> GSKNIVNTSILSIVYKKDDLIDLSRYGAKINIGDRVYYDSIDKNQIKLINLESSTIEVILKNAIVYNSMYENFSTSFWIKIPKYFSKINLNNEYTIINCIENNSGWKVSLNYGEIIWTLQDNKQNIQRVVFKYSQMVNISDYINRWIFVTITNNRLTKSKIYINGRLIDQKPISNLGNIHASNKIMFKLDGCRDPRRYIMIKYFNLFDKELNEKEIKDLYDSQSNSGILKDFWGNYLQYDKPYYMLNLFDPNKYVDVNNIGIRGYMYLKGPRGSVVTTNIYLNSTLYEGTKFIIKKYASGNEDNIVRNNDRVYINVVVKNKEYRLATNASQAGVEKILSALEIPDVGNLSQVVVMKSKDDQGIRNKCKMNLQDNNGNDIGFIGFHLYDNIAKLVASNWYNRQVGKASRTFGCSWEFIPVDDGWGESSL;> MKKHHHHHHGSLVPRGSDVIKPLQSDEYALLTRNVERDKYANFTINFTMENQIHTGMEYDNGRFIGVKFKSVTFKDSVFKSCTFEDVTSVNTYFKNCTFIDTVFDNTDFEPYKFIDSEFKNCSFFHNKTGCQITFD

Botulinum neurotoxins (BoNTs) comprise a family of seven serologically distinct neurotoxin types, designated BoNT/A through BoNT/G, that cause botulism, a rare but potentially fatal paralytic disease, in vertebrates. BoNT molecules are synthesized as single polypeptide chains that are processed into mature toxins by cleavage into two subunits, a 50 kDa light chain (LC) and a 100 kDa heavy chain (HC), that remain connected through a disulfide bond. The HC consists of a 50 kDa N-terminal translocation domain (HN) and a C-terminal receptor-binding domain (HC) of similar size. BoNT/A, BoNT/D, BoNT/E and BoNT/F bind synaptic vesicle protein 2 (SV2)16.

In order to understand how BoNT/A2 can compensate for the missing interactions seen in the BoNT/A1-HC-SV2C-LD complex structure, we determined the crystal structure of SV2C-LD bound to BoNT/A2-HC. As in the previous BoNT/A1-HC – SV2C-LD structures, the quadrilateral β-helix structure formed by SV2C-LD binds to a two-stranded, antiparallel β-sheet on the convex side of BoNT/A2HC. In the extended β-sheet, the interaction is dominated by backbone-to-backbone interactions. BoNT subtype A2 contains a Glu at position 1156 and a Ser at position 1294 and can neither form a cation-π interaction, nor contribute to an overall positive net charge of the receptor binding domain. The structure of the BoNT/A2-HC complex provides an explanation why human SV2C-LD can still bind strongly to toxin subtype A2 despite the pronounced sequence differences in key residues to the A1 subtype. Specific interactions compensate for the lacking cation-π stacking. SV2C-LD His 564 NE2 forms a salt bridge with BoNT/A2-HC Glu 1156 OE2 and a hydrogen bond with BoNT/A2-HC Tyr 1122 OH. Furthermore, Glu 1156 of the toxin engages in an anion- π stacking interaction to Phe 563 of SV2C-LD. In BoNT/A2-HC, residue 1294 is a serine, which does not engage in polar contacts with the receptor. In the BoNT/A2-HC – human SV2C-LD structure, the polypeptide chain in this region forms a long extension that makes a crystal contact with a symmetry-related BoNT molecule.Anion exchanger 2 (AE2) works at high cellular pH to catalyze the exchange between the intracellular HCO3− and extracellular Cl−, thereby maintaining the pH-homeostasis. Here, we determine the cryo-EM structures of human AE2 in five major operating states and one transitional hybrid state. Among those states, the AE2 shows the inward-facing, outward-facing, and intermediate conformations, as well as the substrate-binding pockets at two sides of the cell membrane. In conclusion, given the presently revealed structural models, the AE2 uses NTD as the intracellular pH sensor to mediate the anion-exchanging activities of its TMD, thereby maintaining pH homeostasis.

DIDS is a pan-inhibitor against the anion transporters from SLC4, SLC16, and SLC26A families and chloride channels. Uncertainty remains about the structural basis of the inhibition by DIDS since the electron density for DIDS in the crystal structure of AE1-DIDS is not well resolved, and thus we solved the cryo-EM structure of the human AE2 supplemented with DIDS (hAE2DIDS). The molecular models were thus built in the corresponding EM maps, respectively, using the crystal structure of human AE1 as the starting model. Using similar methods, we further determined EM structures for hAE2 supplemented with inhibitor DIDS (hAE2DIDS) in the presence of HCO3−, and two maps in different conformations were reconstructed, one is named hAE2DIDS with C2 symmetry, the other is hAE2asymmetry with C1 symmetry, at resolutions of 3.08 Å and 3.17 Å respectively. In the EM maps of hAE2 with HCO3− (hAE2NaHCO3) and DIDS (hAE2DIDS), the electron density for NTDs was not well solved, and thus only TMD structures were determined. In the hAE2DIDS structure, an apparent, continuous non-proteinous electron density was identified, and the whole body of the DIDS molecular fit very well. The hAE2DIDS adapts into an outward-facing conformation, and the DIDS molecule lies in the middle of the outer vestibule with one of its isothiocyanato group forming the covalent bond with the ε-amino group of K842, a conserved residue corresponding to the KLIK in AE1. On the other end of DIDS, however, the “Lys-Ser-Thr-Pro” in the TM13 of AE1 is replaced by “Met-Ser-Thr-Ala” in the TM13 of hAE2. The cross-linking between DIDS and hAE2 tightly fixes the inhibitor molecule in the way of the substrates entering/exiting the outer vestibule and thus disrupts the pH-rebalancing capacity of AE2.

>MSSAPRRPAKGADSFCTPEPESLGPGTPGFPEQEEDELHRTLGVERFEEILQEAGSRGGEEPGRSYGEEDFEYHRQSSHHIHHPLSTHLPPDARRRKTPQGPGRKPRRRPGASPTGETPTIEEGEEDEDEASEAEGARALTQPSPVSTPSSVQFFLQEDDSADRKAERTSPSSPAPLPHQEATPRASKGAQAGTQVEEAEAEAVAVASGTAGGDDGGASGRPLPKAQPGHRSYNLQERRRIGSMTGAEQALLPRVPTDEIEAQTLATADLDLMKSHRFEDVPGVRRHLVRKNAKGSTQSGREGREPGPTPRARPRAPHKPHEVFVELNELLLDKNQEPQWRETARWIKFEEDVEEETERWGKPHVASLSFRSLLELRRTLAHGAVLLDLDQQTLPGVAHQVVEQMVISDQIKAEDRANVLRALLLKHSHPSDEKDFSFPRNISAGSLGSLLGHHHGQGAESDPHVTEPLMGGVPETRLEVERERELPPPAPPAGITRSKSKHELKLLEKIPENAEATVVLVGCVEFLSRPTMAFVRLREAVELDAVLEVPVPVRFLFLLLGPSSANMDYHEIGRSISTLMSDKQFHEAAYLADEREDLLTAINAFLDCSVVLPPSEVQGEELLRSVAHFQRQMLKKREEQGRLLPTGAGLEPKSAQDKALLQMVEAAGAAEDDPLRRTGRPFGGLIRDVRRRYPHYLSDFRDALDPQCLAAVIFIYFAALSPAITFGGLLGEKTQDLIGVSELIMSTALQGVVFCLLGAQPLLVIGFSGPLLVFEEAFFSFCSSNHLEYLVGRVWIGFWLVFLALLMVALEGSFLVRFVSRFTQEIFAFLISLIFIYETFYKLVKIFQEHPLHGCSASNSSEVDGGENMTWAGARPTLGPGNRSLAGQSGQGKPRGQPNTALLSLVLMAGTFFIAFFLRKFKNSRFFPGRIRRVIGDFGVPIAILIMVLVDYSIEDTYTQKLSVPSGFSVTAPEKRGWVINPLGEKSPFPVWMMVASLLPAILVFILIFMETQITTLIISKKERMLQKGSGFHLDLLLIVAMGGICALFGLPWLAAATVRSVTHANALTVMSKAVAPGDKPKIQEVKEQRVTGLLVALLVGLSIVIGDLLRQIPLAVLFGIFLYMGVTSLNGIQFYERLHLLLMPPKHHPDVTYVKKVRTLRMHLFTALQLLCLALLWAVMSTAASLAFPFILILTVPLRMVVLTRIFTDREMKCLDANEAEPVFDEREGVDEYNEMPMPV[2x]3-[(4-amino-2-methylpyrimidin-5-yl)methyl]-2-{(S)-hydroxy[(R)-hydroxy(methoxy)phosphoryl]phenylmethyl}-5-(2-{[(R)-hydroxy(phosphonooxy)phosphoryl]oxy}ethyl)-4-methyl-1,3-thiazol-3-ium 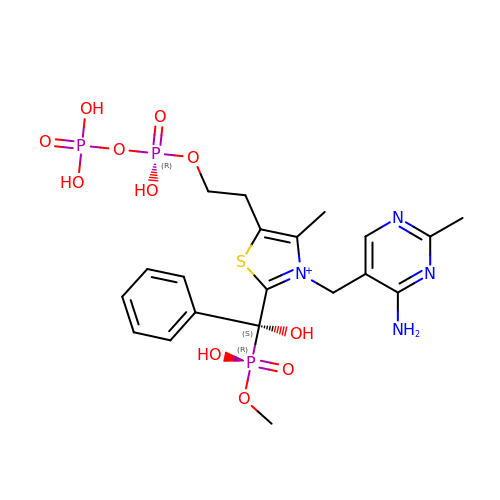| C20 H28 N4 O11 P3 S | NEEQBMRCDKRNBV-FQEVSTJZSA-O> MKITLPKPFFFEGGNRAVLLLHGFTGSSADVRMLGRYLQKHGYTSLAPQYKGHAAPPEELTKTGPADWWQDVLDGYEELKAKGYDEIAVCGLSLGGVMSLRLSMHRPVKAVIPMCAPAYIKSEDVMYAGVTEYAREFKKREGKSVDEIEQEMAVFEPMPTLKDLQALLKETRDSLEDVYAPTLVVQARNDHMINTDSANIIHDGVSALQKELIWYENSGHVITLDKEKETLHQDIHEFLDGLNWSH

Sequence and phylogenetic analyses showed that EaEst2 belongs to the Family XIII group of carboxylesterases. EaEst2 has a broad range of substrate specificities for short-chain p-nitrophenyl (pNP) esters, 1-naphthyl acetate (1-NA), and 1-naphthyl butyrate (1-NB). Its optimal pH is 7.0, losing its enzymatic activity at temperatures above 50 °C. EaEst2 showed degradation activity toward bis(2-hydroxyethyl) terephthalate (BHET), a polyethylene terephthalate degradation intermediate.

The crystal structure of EaEst2 has been determined at a 1.74 Å resolution in the ligand-free form. The structure was refined to an Rwork of 19.6% and an Rfree of 21.3%. The asymmetric unit of the crystal (space group P212121) contained one EaEst2 molecule and 169 water molecules. The overall structure of EaEst2 comprised seven β-strands and 10 α-helices and adopted a classical α/β hydrolase fold in the core domain, which was a twisted β sheet surrounded by α-helices and a cap domain. Three putative catalytic residues, S93, D190, and H220, were located on the β4-α4, β6-α8, and β7-α9 loops, respectively. Notably, the substrate binding pocket of EaEst2 was covered by a cap domain comprising α2-, α5-, and α6-helices, forming a long and narrow shape. Additionally, our sequence analysis revealed that EaEst2 possesses a conserved pentapeptide, GLSLG, in its amino acid sequence from 91–95, including a catalytic Ser residue, which is a typical consensus motif in carboxylesterase Family XIII enzymes. Unlike most carboxylesterases, which are thought to exist as dimers in solution, the functional unit of EaEst2 was determined to be a monomer by size-exclusion chromatography. Collectively, the EaEst2 enzyme can degrade BHET into MHET by cleavage of the ester bond and cannot utilize MHET as a substrate. As a result, we investigated the possible interaction mode between EaEst2 and BHET using computational docking simulations.> HHHHHHMPSSVSWGILLLAGLCCLVPVSLAEDPQGDAAQKTDTSHHDQDHPTFNKITPNLAEFAFSLYRQLAHQSNSTNIFFSPVSIATAFAMLSLGTKADTHDEILEGLNFNLTEIPEAQIHEGFQELLRTLNQPDSQLQLTTGNGLFLSEGLKLVDKFLEDVKKLYHSEAFTVNFGDTEEAKKQINDYVEKGTQGKIVDLVKELDRDTVFALVNYIFFKGKWERPFEVKDTEEEDFHVDQVTTVKVPMMKRLGMFNIQHCKKLSSWVLLMKYLGNATAIFFLPDEGKLQHLENELTHDIITKFLENEDRRSASLHLPKLSITGTYDLKSVLGQLGITKVFSNGADLSGVTEEAPLKLSKAVHKAVLTIDEKGTEAAGAMFLEAIPMSIPPEVKFNKPFVFLMIEQNTKSPLFMGKVVNPTQK

α1-Antitrypsin is the most abundant antiprotease in the human circulation. It is also the archetypal member of the serpin (serine protease inhibitor) superfamily of proteins. Serpins are characterized by a metastable native fold consisting of nine α-helices (A–I) and three β-­pleated sheets (A–C). A propensity to undergo stabilizing conformational change involving expansion of β-sheet A is utilized in the structural transitions required for protease inhibition.

We have now solved the highest resolution (1.8 Å) crystal structure of α1-antitrypsin. A new 1.8 Å resolution structure of α1-antitrypsin demonstrates structural variability within this site, with associated fluctuations in its upper and lower entrance grooves and ligand-binding characteristics around the innermost stable enclosed hydrophobic recess. The increased detail provides insight into the mechanism of β-sheet A expansion by delineating the hydration of a relatively hydrophobic environment around the highly conserved Trp194 residue, rendering the initial loop insertion site conformationally labile. These data nicely explain findings from previous tryptophan fluorescence studies of conformational change during polymerization. Occupancy of alternative rotameric orientations for Val216 and Ile340 became apparent during refinement. These are found on β-­strand s4C and in the hinge region between β-strand s5A and the reactive loop. Previous structures of native wild-­type α1-antitrypsin have indicated the presence of zero, one or two waters in this region. Fascinatingly, the intrinsic fluorescence spectrum of α1-antitrypsin reports the formation of both the intermediate and polymer during polymerization by a small blue shift and increased intensity attributable to Trp194. Moreover, comparison with 2.0 Å resolution structures characterizes variation in the conformational dynamics of the allosteric pocket in solution.> GMSENKKKFDKKGAKNMDEISKTLFAPIYPIIAENIINRFGITAGTCIDIGSGPGALSIALAKQSDFSIRALDFSKHMNEIALKNIADANLNDRIQIVQGDVHNIPIEDNYADLIVSRGSVFFWEDVATAFREIYRILKSGGKTYIGGGFGNKELRDSISAEMIRKNP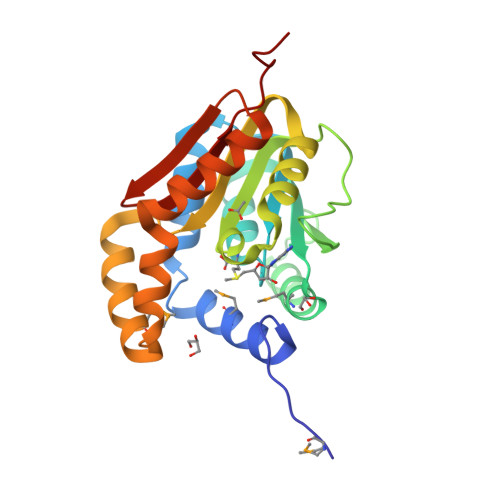DWKEFNRKNISQENVERFQNVLDEIGISSYEIILGDEGFWIIISKTDQEVI>[2x]AETSSATTAQQMPSLAPMLEKVMPSVVSINVEGSTTVNTPRMPRNFQQFFG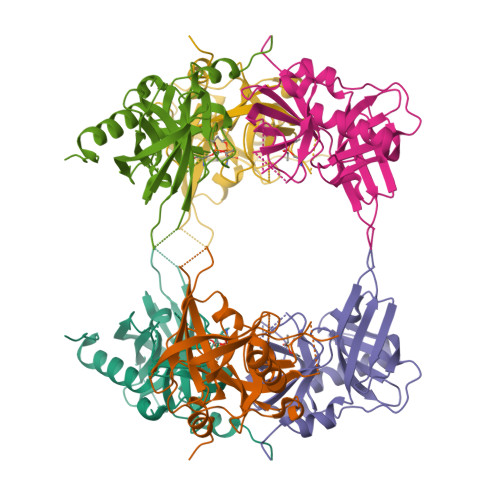DDSPFCQEGSPFQSSPFCQGGQGGNGGGQQQKFMALGSGVIIDADKGYVVTNNHVVDNATVIKVQLSDGRKFDAKMVGKDPRSDIALIQIQNPKNLTAIKMADSDALRVGDYTVAIGNPFGLGETVTSGIVSALGRSGLNAENYENFIQTDAAINRGNSGGALVNLNGELIGINTAILAPDGGNIGIGFAIPSNMVKNLTSQMVEYGQVKRGELGIMGTELNSELAKAMKVDAQRGAFVSQVLPNSSAAKAGIKAGDVITSLNGKPISSFAALRAQVGTMPVGSKLTLGLLRDGKQVNVNLELQQSSQNQVDSSSIFNGIEGAEMSNKGKDQGVVVNNVKTGTPAAQIGLKKGDVIIGANQQAVKNIAELRKVLDSKPSVLALNIQRGDSTIYLLMQRSHHHHHH In mammals, the canonical Hippo pathway contains a core kinase cascade, formed by STE20-like MST1/2 kinases, Large Tumor Suppressor LATS1/2 kinases, the WW-domain containing scaffold protein Salvador (SAV1) and the adaptor protein MOB1. MST1/2 contain an N-terminal kinase domain and a C-terminal coiled-coil SARAH domain, which are separated by a flexible linker. MST1 and MST2 can each form a constitutive homodimer through the SARAH domain, and kinase activation is achieved by trans-autophosphorylation of the activation loop (T183 for MST1 and T180 for MST2). In this study, using a combination of biochemical, structural, and cell biological experiments, we establish the PP2A complex, STRIPAKSLMAP, as a key negative regulator of Hippo signaling in human cells, and show that SAV1 promotes MST1/2 activation through antagonizing the STRIPAKSLMAP PP2A phosphatase activity.

To understand how SLAMP FHA recognized phospho-MST2, we obtained crystals of SLMAP FHA bound to the pT378-MST2371-401 peptide (pMST2 hereafter for simplicity) that diffracted to 1.55 Å resolution. We determined the structure of SLMAP FHA–pMST2 by molecular replacement using apo-SLMAP FHA as the search model. In the SLMAP FHA–pMST2 structure, the FHA domain adopts a conformation virtually identical to that of free SLMAP FHA with an RMSD of 0.33 Å for all atoms, indicating that binding of pMST2 does not appreciably alter the conformation of the FHA domain. Only six residues of pMST2 (D376GpTMKR381) have clear electron density, and bind to a surface formed by residues from the β3-β4, β4-β5, β6-β7, and β10-β11 loops of SLMAP FHA. The pT378 residue binds at a highly positively charged pocket, with the phosphate group making favorable electrostatic interactions with side chain or main chain atoms from R32, S52, R53 and S75 of SLMAP. M379 inserts into an adjacent hydrophobic pocket on SLMAP. R381 makes hydrophobic and electrostatic interactions with side chains from V107 and V109, and main chain from D108 of SLMAP, respectively, indicating that a positively charged residue is preferred at this position. D376 forms two hydrogen bonds with R53 of SLMAP. G377 forms a 90˚ turn to allow D376 to make favorite contacts with R53 of SLMAP. Our structure thus suggests that SLMAP FHA prefers binding to a phospho-threonine peptide with a consensus sequence of E/D-G-pT-M-x-R/K. Consistent with this prediction, the pT325-MST2320-329 and pT336-MST2331-340 peptides that do not fully conform to this consensus bind to SLMAP FHA with lower affinities.

>[2x]MPSALAIFTCRPNSHPFQERHVYLDEPIKIGRSVARCRPAQNNATFDCKVLSRNHALVWFDHKTGKFYLQDTKSSNGTFINSQRLSRGSEESPPCEILSGDIIQFGVDVTENTRKVTHGCIVSTIKLFLPDGMEARLRSD;>EEEDGTMKRN[2x]>[2x]MNLFQTVFTGSKQALAAAEGIVKQAVDEKGRDYKVAFPDTAYSLPVIFAATGKKITNVGELEGALDIVRSLIVEEEMLDKLLNSGLATAVAAEIIEAAKYVLSDAPYAEPCVGFISDPIIRSLGVPLVTGDIPGVAVILGECPDSETAAKIIKDYQSKGLLTCLVGKVIDQAIEGKVKMGLDLRVIPLGYDVTSVIHVVTIAIRAALIFGGIKGGQLNDILKYTAERVPAFVNAFGPLSELVVSAGAGAIALGFPVLTDQVVPEVPTLLLTQKDYDKMVKTSLEARNIKIKITEIPIPVSFAAAFEGER;>MEEKAKSIDQATLQLLDKAKQDGVETVWDRKADMKVQCGFGSAGVCCRNCSMGPCRVSPVPGKGVERGICGATADVIVSRNFARMVAAGTAAHSDHGRSIALSLYHTSKDGDIKVKDENKLKEVAKSFNVETEGRDIYDIAHDVAKEGLSNYGKQLGEVTLPPSLPEKRKELWRK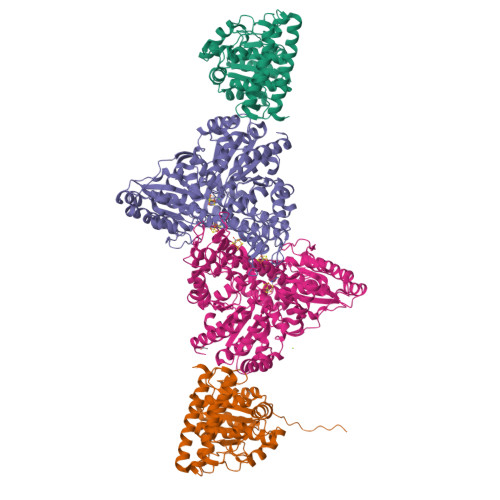LGVYPRAVDREIAAVMHSTHIGCNADAEAMIKMSMRCSLTDGWMGSFMGTEFSDIMFGTPHSIDTEANLGVLEKNSVNVVLHGHEPLLSEMVVEAASDPELVELAKSVGADGINLCGMCCTGNEVSMRHGIKIAGNFMQQELAVVTGAVDGLIVDVQCIMPALAKLSKSYHTKFITTSPKAHITDSIYMEFDEENPLDSAKKILKEAILNFKNRDQSKVMIPELKCKAILGYSVEEIINKLDKVVNTQIGPMQTVKPLADVLVSGVLRGAAAVVGCNNPKVVQDSAHIETIKGLIKNDVIVVVTGCAAQAAAKYGLLQKEAAEKYAGPGLATVCKLVDIPPVLHMGSCVDISRILDLVGRVANLLGVDMSDLPVAGVAPEWMSEKAVAIGTYVVTSGIDTWLGVAPPVTGGPEVVDILTNKMEDWVGAKFFIETDPHKAVEQIVNRMNEKRKKLGI[2x]>MARSKDVTPWDVNINNEEGINYNKLIKEFGCSKITENHIKRIEKLTNSKAHHFIRRGIFFSHRDLDFLLNYYEQHKCFYIYTGRGPSSLSMHLGHLIPFYFCKYLQEAFNVPLVIQLSDDEKYLFNQNYSLEYINTLTNENVKDIISVGLNPELTFIFKNTEYAGYLYPTVLSIHKKTTLNQSMNVFGFNHSDNIGKISYPSFQIAPCFSQCFPNFLGKNIPCLVPQGIDQDPYFRLSRDIAVKMALHKPVVVHSVFMPGLQGVNSKMSSTKKKKDDNGKSNSTFDHNNSVIFLTDTPEQIKNKINKYAFSGGGTTIQEHREKGGNLDKDISYQYLRYLLEDDNKLNEIGEKYKKGEMLSGEIKKILIDVLTELVLKHQEKKKSLTDEEISYFFDPNKPSLQKFKNMENLYFQGHHHHHH[4x]

Tryptophanyl-tRNA synthetase (WRS) is a class I aaRS and all members of this class are characterized by a Rossmann-fold catalytic domain whose active site is recognizable by the presence of consensus sequences HIGH and KMSKS. The Plasmodium falciparum genome contains two copies of tryptophanyl-tRNA synthetase – a cytoplasmic version (hereafter Pf-WRS, Plasmodb ID PF13_0205) and an apicoplastic one (hereafter Pf-WRSapi, Plasmodb ID PFL2485c). Pf-WRS has an unusual N-terminal appendage of an Ala-X like domain (AXD) which we show is necessary for enzymatic activity. Here, we present crystal structure of malaria parasite Plasmodium falciparum cytoplasmic tryptophanyl-tRNA synthetase (Pf-WRS) catalytic domain (AAD) at 2.6 Å resolution in complex with L-tryptophan.

However, a construct encoding for the catalytic domain (AAD) of Pf-WRS (228–632) crystallized in the presence of L-tryptophan (L-Trp). These crystals diffracted to 2.6 Å resolution and belong to space group P21 with two dimers of Pf-WRS AAD in the asymmetric unit (solvent content of ∼56%). Structure of Pf-WRS AAD (monomer) consists of 6 β strands and 19 α helices and each monomer harbors the N-terminal aminoacylation domain (residues 228–496) and an anticodon-binding domain (residues 497–629). Well defined electron density was observed for the bound L-Trp in the active site of all four chains. We could only observe clear electron density for the bound L-Trp but not for ATP although crystals were grown in the presence of both. In Pf-WRS AAD crystal structure residues 482–512 include the ATP-binding motif KMSST which is completely disordered. However, the KMSST loop in Pf-WRS has a fifteen residues insertion immediately following this key motif. A potassium ion (K+ ion) was observed at the dimer interface and the coordination distances between this ion, protein atoms and water molecules are in ranges of 2.8–3.6 Å. Residues from both monomers contribute to the ligation of the bound K+ ion, which to our knowledge has not been reported for any WRS crystal structure so far. Sequence identity between parasite and human enzyme counterparts is ∼55% and the overall fold of Pf-WRS is hence very similar to Hs-WRS.>IEEEDVICDGCNGPVVGTRYKCSVCPDYDLCSVCEGKGLHRGHTKLAFPSPFGHLSE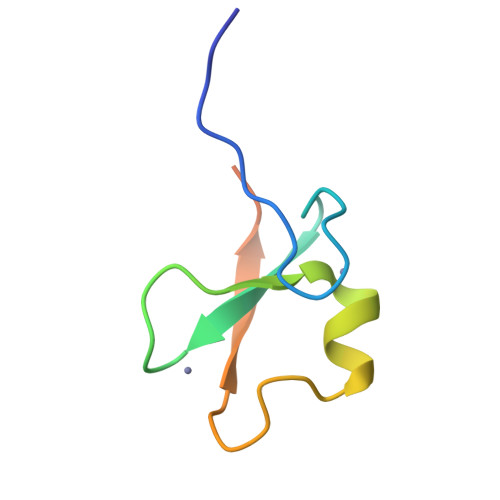GFS[2x]>MLPALIGISGHEVGAEEEAAIRRLQPAGFILFSRNIDSVEQVRGLTESLRKLCLHHPVIAVDQEGGRVVRTASLGLNLPSPASLARLGSVGGIVELGAVTALALRYLGVNLNFAPVLDICHDPSAANALPGRCWGDNAQDVISRGGVYASNLRRGGVQSCGKHFPGMGRALADPHFSLPVIGLDERELFKTDLLPFLALCPALSSIMSAHIMLPQIDPDYPATLSERVIRGLLRDRLGFRGVVFTDDLCMGAITTQYSPDDAAFLSLKAGCDLPLICHDPLPWLDGLASRQESLNAYDRWD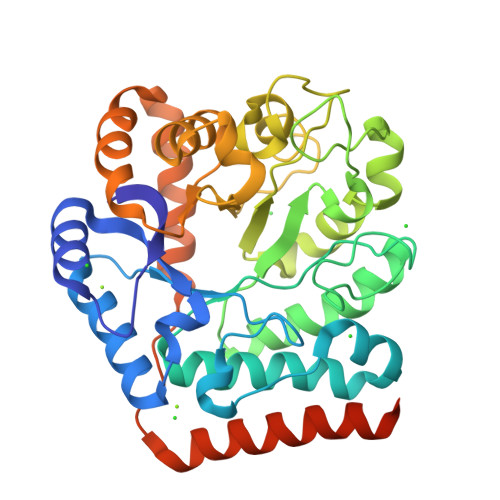SFKRVEKLSDSLCFPFPEKASLWDSCLRRAEALCRLEEDGREKLPSSPVQKYLEHHHHHH[2x]> MTPKTETPVGALIKKFFPGKRFQKNYLKDAGKKLKREGEAAAVEYLSGKQEDHPANFCPPAKVNILAQSRPLSEWPINLVSKGVQEYVYGLTAAEREANGDFGTSRKSLDRWFARTGVPTHGYTTVQGLNLILRHTFNRYDGVIKKVETRNEKRRSKATRINVSREADGLPPIEAEPEETAFGPDGKLKERPGINPSIYCYQQVSPVPYNPAKHPALPFSGVDPGAPLPLGTPNRLSIPKGQPGYVPEWQRPHLSTKNKRIRKWYARANWRRKPGRKSVLDEAKLKEAALKEAIPIIVTIGKDWIVMDARGLLRAVYWRGIAKPGLSLKELLGFFSGDPVLDPKRGIATFTFKLGAVAVHSRKPTRGKKSKELLLSMTAEKPHVGLVAIDLGQTNPVAAEFSRVKREGETLQAEPLGQIVLPDDLVKDLTRYRRAWDATEEQIKAEAIVQLPEECRAEVVKVNQMSAEETKHLILDRGVSGDLPWEKMTSNTTFISDHLLAKGVTDQVFFEKKSKGKKKGTETVKRKDYGWVKLLRPRLSQETRKAVNDKTWELKRASTEYVRLSRRKTELARRCVNYIVRETKRWTQCEDIAIVIEDLNVRFFHGSGERPDGWDNFFISKRENRWFIQVLHKAFSDLALHRGLPVIEANPARTSITCIRCGHCDRNNRHGEMFLCLSCNDLRHADREIATRNLTRVAVTGEMIPRRIEPGEQSGDTKKARSARKGKKAVISKREAA

By searching the environmental metagenomic sequences with the conserved Ruvc nuclease domain of CasΦ2 (Cas12j-2) proteins, we identified a new hypercompact type V CRISPR-Cas system derived from Caudoviricetes, named Cas12j-SF05 (or CasΦ-SF05), which phylogenetically belongs to the Cas12j family. The CRISPR locus contains the Cas12j-SF05 gene encoding a 737 aa protein, and a CRISPR array that consists of 36 bp repeating sequences separated by 35–38 bp spacer sequences. The results showed that Cas12j-SF05crRNA has a preference for a 5′-TBN-3′ PAM (B is for T, C, or G) for target dsDNA cleavage. Sanger-sequencing of the target plasmids cleaved by Cas12j-SF05crRNA revealed the generation of double-stranded breaks with staggered 5′ overhangs of 7 nt, similar to the cleavage pattern observed in other Ca12j family memebers.

To investigate the molecular mechanisms of Cas12j-SF05 crRNA recognition and cleavage of its dsDNA target, we reconstructed the dsDNA-bound Cas12j-SF05crRNA complex by incubating the Cas12j-SF05crRNA with a target dsDNA containing a ‘TTC’ PAM for 30 min. The complex was presumed to be in a post-cleavage state, as the target dsDNA would have been cleaved by the Cas12j-SF05crRNA during the incubation period. We determined the cryo-EM structure of Cas12j-SF05crRNA-dsDNA ternary complex at a resolution of 3.1 Å. The Cas12j-SF05 adopted a typical bilobed architecture, consisting of the recognition (Rec) and nuclease (Nuc) lobes, which resembles CasΦ-2 (Cas12j-2) with an RMSD of 1.534 Å over 364 Cα atoms. The Rec lobe contains several domains, including the PAM-Interacting domain (PI), the oligonucleotide binding domain (OBD), and two α-helical bundle domains (RecI and RecII). The Nuc lobe contains a C-terminal RuvC endonuclease domain (RuvC) and an invisible zinc finger domain (ZR), which is responsible for cleaving the target dsDNA. In our determined Cas12j-SF05crRNA-dsDNA ternary complex, we observed a 36-nt crRNA bound to a 22-nt traceable TS and 7-nt traceable NTS of the 55-bp dsDNA target. We could not observe the density of the PI domain, but we did observe that the bases of A-3 and A-2 of the TS, which are complementary to the 5′-TTC-3′ PAM, are recognized by two highly conserved glutamine residues Q202 in the OBD domain and Q127 in the RecI domain. Upon PAM recognition, the residue S336 in OBD domain facilitates the unwinding of target dsDNA by binding to the backbone phosphate group of G-1 (right inset). The subsequently formed crRNA-TS duplex is further stabilized by a series of sequence-nonspecific interactions mediated by a long α helix and an adjacent loop region in RecI domain (right inset).> MGSSHHHHHHSQDPAEKQKHDGRVKIGHYVLGDTLGVGTFGKVKIGEHQLTGHKVAVKILNRQKIRSLDVVGKIKREIQNLKLFRHPHIIKLYQVISTPTDFFMVMEYVSGGELFDYICKHGRVEEMEARRLFQQILSAVDYCHRHMVVHRDLKPENVLLDAHMNAKIADFGLSNMMSDGEFLRTSCGSPNYAAPEVISGRLYAGPEVDIWSCGVILYALLCGTLPFDDEHVPTLFKKIRGGVFYIPEYLNRSVATLLMHMLQVDPLKRATIKDIREHEWFKQGLPSYLFPEDPSYDANVIDDEAVKEVCEKFECTESEVMNSLYSGDPQDQLAVAYHLIIDNRRIMNQASEFYLASSPPSGSFMDDSAMHIPPGLKPHPERMPPLIADSPKARCPLDALNTTKPKSLAVKKAKWHLGIRSQSKPYDIMAEVYRAMKQLDFEWKVVNAYHLRVRRKNPVTGNYVKMSLQLYLVDNRSYLLDFKSIDDEVVEQRSGSSTPQRSCSAAGLHRPRSSFDSTTAESHSLSGSLTGSLTGSTLSSVSPRLGSHTMDFFEMCASLITTLAR;> MGNTTSDRVSGERHGAKAARSEGAGGHAPGKEHKIMVGSTDDPSVFSLPDSKLPGDKEFVSWQQDLEDSVKPTQQARPTVIRWSEGGKEVFISGSFNNWSTKIPLIKSHNDFVAILDLPEGEHQYKFFVDGQWVHDPSEPVVTSQLGTINNLIHVKKSDFEVFDALKLDSMESSETSCRDLSSSPPGPYGQEMYAFRSEERFKSPPILPPHLLQVILNKDTNISCDPALLPEPNHVMLNHLYALSIKDSVMVLSATHRYKKKYVTTLLYKPI;> MADLNWETVISSDSSPAVENEHPQETPESNNSVYTSFMKSHRCYDLIPTSSKLVVFDTSLQVKKAFFALVTNGVRAAPLWDSKKQSFVGMLTITDFINILHRYYKSALVQIYELEEHKIETWREVYLQDSFKPLVCISPNASLFDAVSSLIRNKIHRLPVIDPESGNTLYILTHKRILKFLKLFITEFPKPEFMSKSLEELQIGTY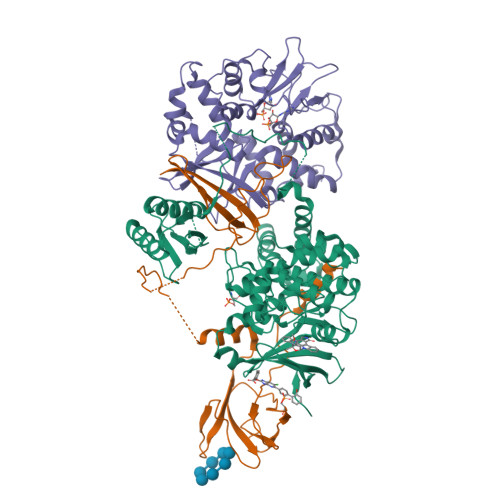ANIAMVRTTTPVYVALGIFVQHRVSALPVVDEKGRVVDIYSKFDVINLAAEKTYNNLDVSVTKALQHRSHYFEGVLKCYLHETLETIINRLVEAEVHRLVVVDENDVVKGIVSLSDILQALVLTGGEKKP> GPHMKHPLQNRWALWFFKNDKSKTWQANLRLISKFDTVEDFWALYNHIQLSSNLMPGCDYSLFKDGIEPMWEDEKNKRGGRWLITLNKQQRRSDLDRFWLETLLCLIGESFDDYSDDVCGAVVNVRAKGDKIAIWTTECENREAVTHIGRVYKERLGLPPKIVIGYQSHADTATKSGSTTKNRFVV;> GPHMTRIIYDRKF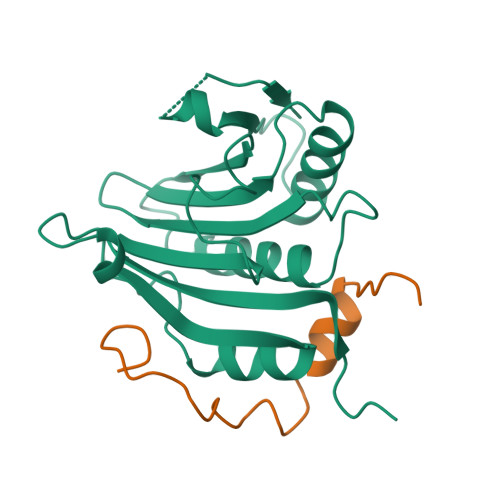LMECRNSPVTKTPPRDLPTIPGVTS> LMPDSGAVFTFGKSKFAENNPGKFWFKNDVPVHLSCGDEHSAVVTGNNKLYMFGSNNWGQLGLGSKSAISKPTCVKALKPEKVKLAACGRNHTLVSTEGGNVYATGGNNEGQLGLGDTEERNTFHVISFFTSEHKI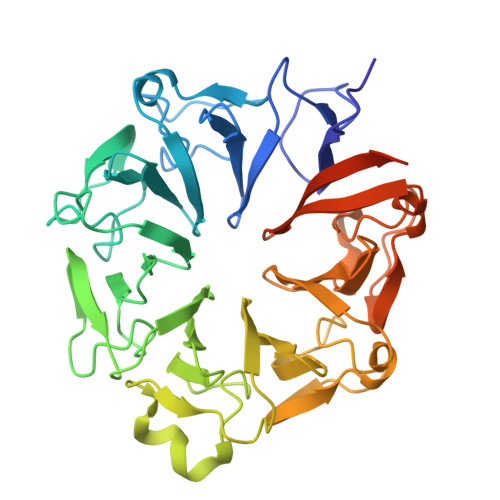KQLSAGSNTSAALTEDGRLFMWGDNSEGQIGLKNVSNVCVPQQVTIGKPVSWISCGYYHSAFVTTDGELYVFGEPENGKLGLPNQLLGNHRTPQLVSEIPEKVIQVACGGEHTVVLTENAVYTFGLGQFGQLGLGTFLFETSEPKVIENIRDQTISYISCGENHTALITDIGLMYTFGDGRHGKLGLGLENFTNHFIPTLCSNFLRFIVKLVACGGCHMVVFAAPHPRRPPAYVEQKLISEEDLNSAVDHHHHHH> SPVVVEREREEFVGFFPQIVRDLTEDGIGHPEVGDAVARLKEVLQYNAPGGKCNRGLTVVAAYRELSGPGQKDAESLRCALAVGWCIELFQAFFLVADDIMDQSLTRRGQLCWYKKEGVGLDAINDSFLLESSVYRVLKKYCRQRPYYVHLLELFLQTAYQTELGQMLDLITAPVSKVDLSHFSEERYKAIVKYKTAFYSFYLPVAAAMYMVGIDSKEEHENAKAILLEMGEYFQIQDDYLDCFGDPALTGKVGTDIQDNKCSWLVVQCLQRVTPEQRQLLEDNYGRKEPEKVAKVKELYEAVGMRAAFQQYEESSYRRLQELIEKHSNRLPKEIFLGLAQK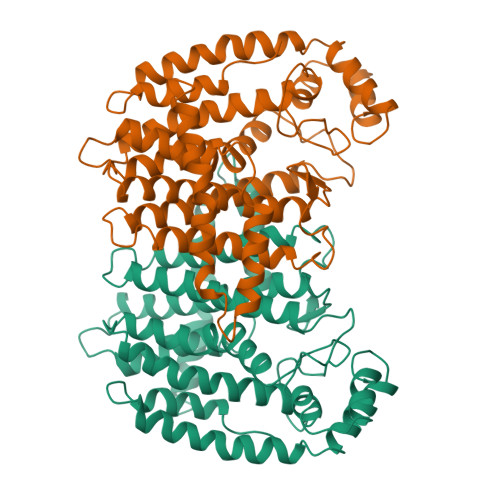IYKRQK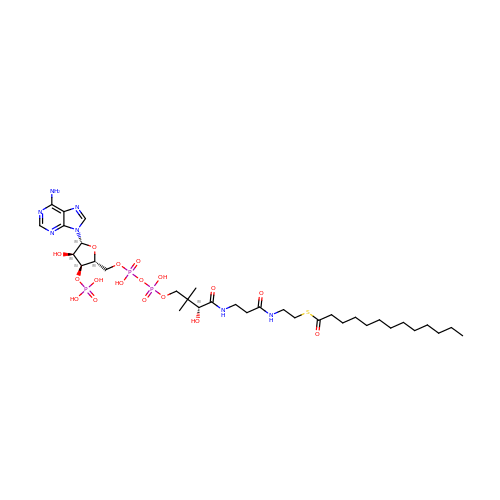~{S}-[2-[3-[[(2~{R})-4-[[[(2~{R},3~{S},4~{R},5~{R})-5-(6-aminopurin-9-yl)-4-oxidanyl-3-phosphonooxy-oxolan-2-yl]methoxy-oxidanyl-phosphoryl]oxy-oxidanyl-phosphoryl]oxy-3,3-dimethyl-2-oxidanyl-butanoyl]amino]propanoylamino]ethyl] tridecanethioate | C34 H60 N7 O17 P3 S | TZKUYUHMJHEXOQ-QYIUPXBKSA-N>SNAMNIEIKDTLISEEQLQEKVKELALQIERDFEGEEIVVIAVLKGSFVFAADLIRHIKNDVTIDFISASSYGNQT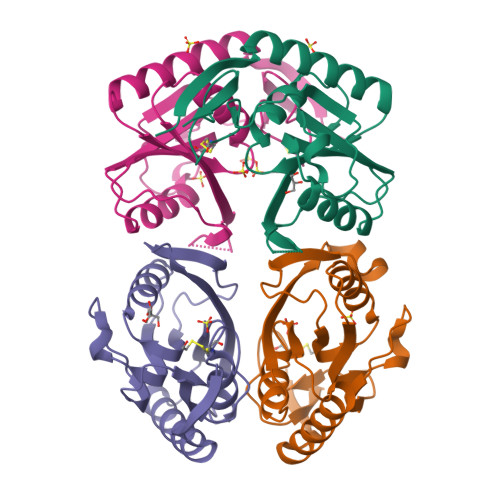ETTGKVKLLKDIDVNITGKNVIVVEDIIDSGLTLHFLKDHFFMHKPKALKFCTLLDKPERRKVDLTAEYVGFQIPDEFIVGYGIDCAEKYRNLPFIASVVTEESYNLKSR[4x]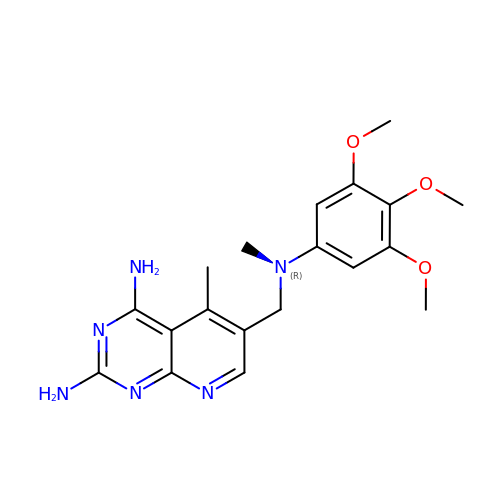2,4-DIAMINO-5-METHYL-6-[(3,4,5-TRIMETHOXY-N-METHYLANILINO)METHYL]PYRIDO[2,3-D]PYRIMIDINE | C19 H24 N6 O3 | PEGMMEYCSOZKIT-UHFFFAOYSA-N>[7x]MTSRDGYQWTPETGLTQGVPSLGVISPPTNIEDTDKDGPWDVIVIGGGYCGLTATRDLTVAGFKTLLLEARDRIGGRSWSSNIDGYPYEMGGTWVHWHQSHVWREITRYKMHNALSPSFNFSRGVNHFQLRTNPTTSTYMTHEAEDELLRSALHKFTNVDGTNGRTVLPFPHDMFYVPEFRKYDEMSYSERIDQIRDELSLNERSSLEAFILLCSGGTLENSSFGEFLHWWAMS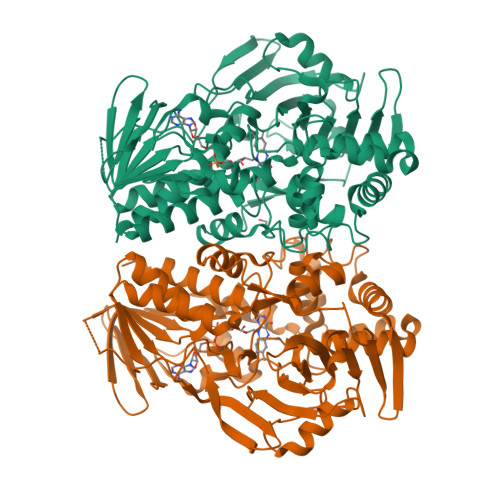GYTYQGCMDCLMSYKFKDGQSAFARRFWEEAAGTGRLGYVFGCPVRSVVNERDAARVTARDGREFVAKRVVCTIPLNVLSTIQFSPALSTERISAMQAGHVSMCTKVHAEVDNKDMRSWTGIAYPFNKLCYAIGDGTTPAGNTHLVCFGTDANHIQPDEDVRETLKAVGQLAPGTFGVKRLVFHNWVKDEFAKGAWFFSRPGMVSECLQGLREKHGGVVFANSDWALGWRSFIDGAIEEGTRAARVVLEELGTKREVKARL;> MTSRDGYQWTPETGLTQGVTSLGVISPPTNIEDTDKDGPWDVIVIGGGYCGLTATRDLTVAGFKTLLLEARDRIGGRSWSSNIDGYPYEMGGTWVHWHQSHVWREITRYKMHNALSPSFNFSRGVNHFQLRTNPTTSTYMTHEAEDELLRSALHKFTNVDGTNGRTVLPFPHDMFYVPEFRKYDEMSYSERIDQIRDELSLNERSSLEAFILLCSGGTLENSSFGEFLHWWAMSGYTYQGCMDCLMSYKFKDGQSAFARRFWEEAAGTGRLGYVFGCPVRSVVNERDAARVTARDGREFVAKRVVCTIPLNVLSTIQFSPALSTERISAMQAGHVSMCTKVHAEVDNKDMRSWTGIAYPFNKLCYAIGDGTTPAGNTHLVCFGTDANHIQPDEDVRETLKAVGQLAPGTFGVKRLVFHNWVKDEFAKGAWFFSRPGMVSECLQGLREKHGGVVFANSDWALGWRSFIDGAIEEGTRAARVVLEELGTKREVKARL>GMSIIDLTKLEQKVATMWDSILTNSPFIHEVLDGKATKALYAIYMTETYHYTKHNAKNQALVGIMGKDLPGKYLSFCFHHAHEEAGHELMALSDIASIGFDREDVLSSKPLPATETLIAYLYWISATGNPVQRLGYSYWAENVYGYIDPVLKAIQSTLDLTPQSMKFFIAHSKIDAKHAEEVNEMLHEVCKTQEDVDSVVAVMENSLVLTARILDDVW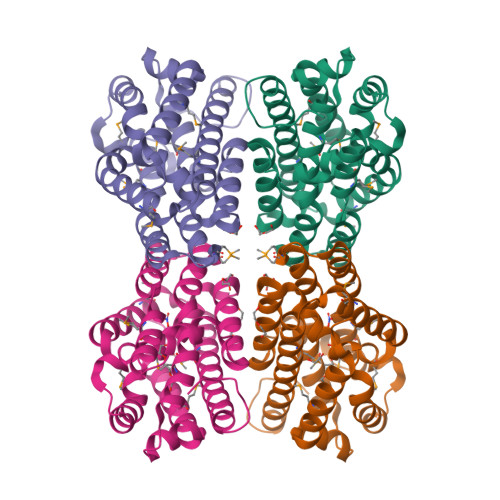KEYQLFQSGASDRYAFLRDNA[2x]N-[4-(1-BENZYLCARBAMOYL-2-METHYL-PROPYLCARBAMOYL)-1-(3,5-DIFLUORO-PHENOXYMETHYL)-2-HYDROXY-4-METHOXY-BUTYL]-5-(METHANESULFONYL-METHYL-AMINO)-N'-(1-PHENYLETHYL)-ISOPHTHALAMIDE | C43 H51 F2 N5 O9 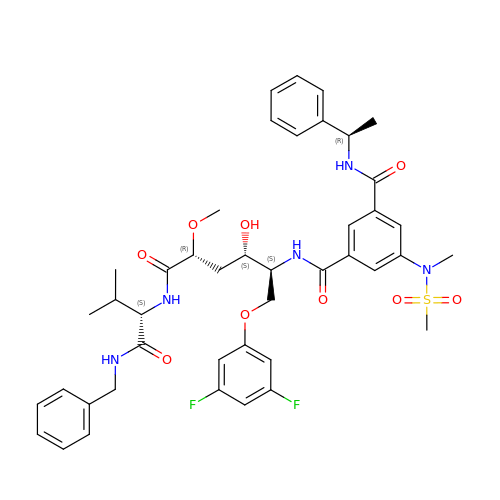S | IEIHXPJWOSDLBU-VWMOWEEZSA-N>[2x]SVIEKLRKLEKQARKQGDEVLVMLARMVLEYLEKGWVSEEDADESADRIEEVLKK

The design of proteins that bind to a specific site on the surface of a target protein using no information other than the three-dimensional structure of the target remains a challenge. Here we describe a general solution to this problem that starts with a broad exploration of the vast space of possible binding modes to a selected region of a protein surface, and then intensifies the search in the vicinity of the most promising binding modes. We demonstrate the broad applicability of this approach through the de novo design of binding proteins to 12 diverse protein targets with different shapes and surface properties. Biophysical characterization shows that the binders, which are all smaller than 65 amino acids, are hyperstable and, following experimental optimization, bind their targets with nanomolar to picomolar affinities.

Unlike antibodies, the designed proteins are soluble when expressed in E. coli at high levels and are thermostable, and hence could form the basis for a next generation of lower cost protein therapeutics.N-[3-(acetylamino)phenyl]-5-{(2E)-2-[(4-methoxyphenyl)methylidene]hydrazino}-3-methyl-1H-pyrazole-4-carboxamide 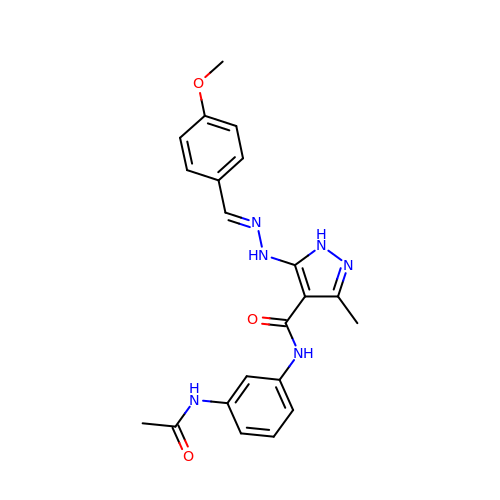| C21 H22 N6 O3 | NIZPETVEBKMXKW-WSDLNYQXSA-N>[8x]EERPLVFLCSGCRRPLGDSLSWVASQ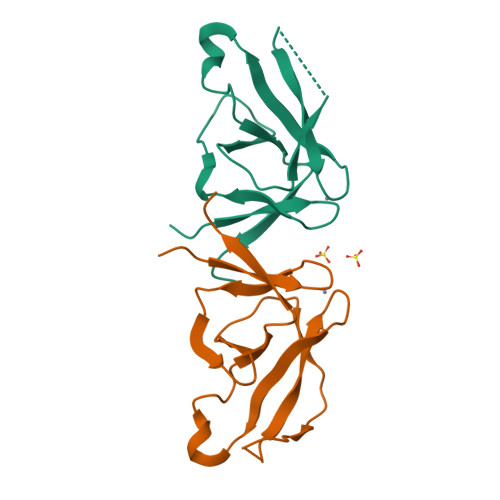EDTNCILLRCVSCNVSVDKEQKLSKREKENGCVLETLCCAGCSLNLGYVYRCTPKNLDYKRDLFCLSVEAIESYVLGSSEKQIVSEDK> MTDQAFVTLTTNDAYAKGALVLGSSLKQHRTTRRLVVLATPQVSDSMRKVLETVFDEVIMVDVLDSG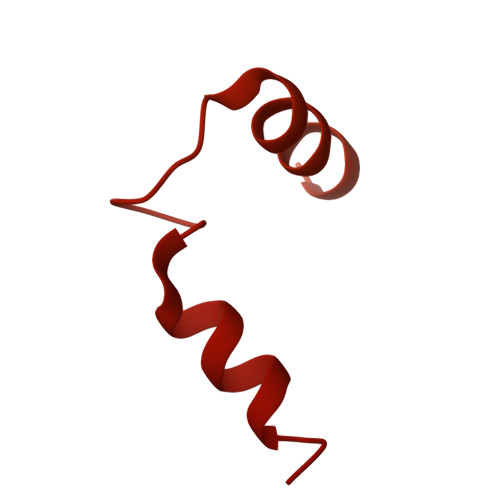DSAHLTLMKRPELGVTLTKLHCWSLTQYSKCVFMDADTLVLANIDDLFDREELSAAPDPGWPDCFNSGVFVYQPSVETYNQLLHLASEQGSFDGGDQGILNTFFSSWATTDIRKHLPFIYNLSSISIYSYLPAFKVFGASAKVVHFLGRVKPWNYTYDPKTKSVKSEAHDPNMTHPEFLILWWNIFTTNVLPLLQQFGLVKDTCSYVNVLSDLVYTLAFSCGFCRKEDVSGAISHLSLGEIPAMAQPFVSSEERKERWEQGQADYMGADSFDNIKRKLDTYLQ> GPPKVPPGPNITTNYNGKWLTARATWYGQPNGAGAPDNGGACGIKNVNLPPYSGMTACGNVPIFKDGKGCGSCYEVRCKEKPECSGNPVTVYITDMNYEPIAPYHFDLSGKAFGSLAKPGLNDKIRHCGIMDVEFRRVRCKYPAGQKIVFHIEKGCNPNYLAVLVKYVADDGDIVLMEIQDKLSAEWKPMKLSWGAIWRMDTAKAL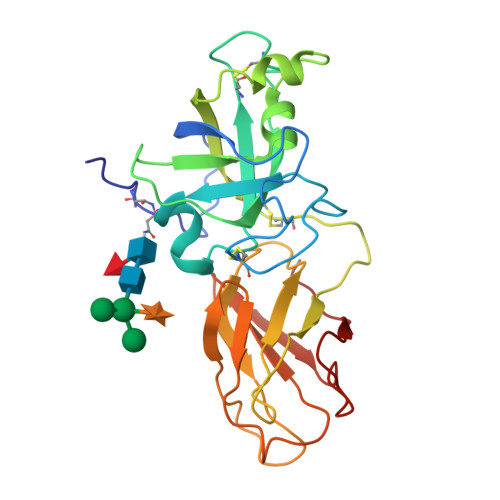KGPFSIRLTSESGKKVIAKDVIPANWRPDAVYTSNVQFY> GSPEFMDDIFTQCREGNAVAVRLWLDNTENDLNQGDDHGFSPLHWACREGRSAVVEMLIMRGARINV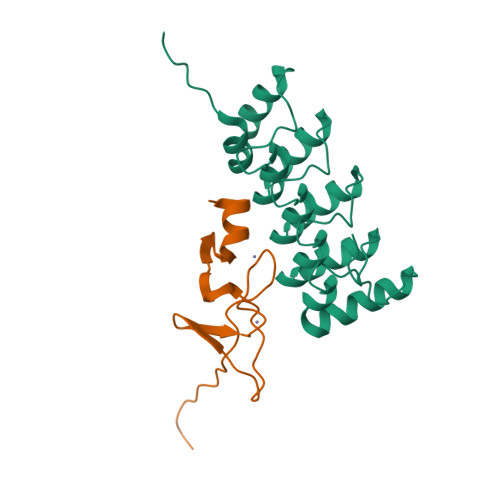MNRGDDTPLHLAASHGHRDIVQKLLQYKADINAVNEHGNVPLHYACFWGQDQVAEDLVANGALVSICNKYGEMPVDKAKAPLRELLRERAEKMGQNLNRIPYKDTFWKGTTR;> SENLYFQGSANAVCQRCQARFSPAERIVNSNGELYHEHCFVCAQCFRPFPEGLFYEFEGRKYCEHDFQMLFA> MRYEVNIVANPNLDQS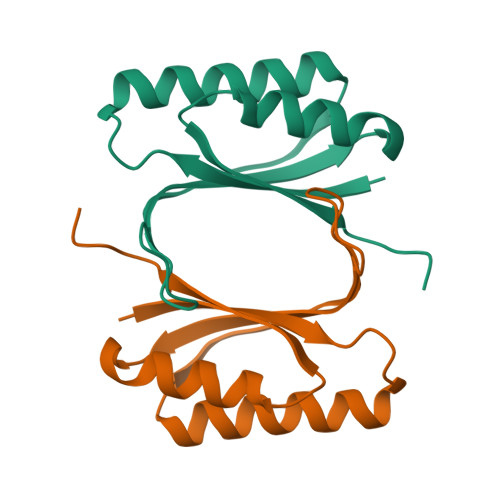QLALEKEIIQRALENYGARVEKVEELGLRRLAYPIAKDPQGYFLWYQVEMPEDRVNDLARELRIRDNVRRVMVVASTTPGRYEVN> S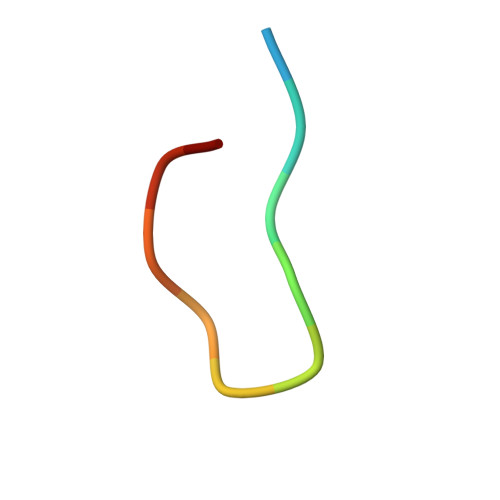DKENFWGMAVA>EPVAVVGISCRVPGARDPREFWELLAAGGQAVTDVPADRWNAGDFYDPDRSAPGRSNSRWGGFIEDVDRFDAAFFGISPREAAEMDPQQRLALELGWEALERAGIDPSSLTGTRTGVFAGAIWDDYATLKHRQGGAAITPHTVTGLHRGIIANRLSYTLGLRGPSMVVDSGQSSSLVAVHLACESLRRGESELALAGGVSLNLVPDSIIGASKFGGLSPDGRAYTFDARANGYVRGEGGGFVVLKRLSRAVADGDPVLAVIRGSAVNNGGAAQGMTTPDAQAQEAVLREAHERAGTAPADVRYVELHGTGTPVGDPIEAAALGAALGTGRPAGQPLLVGSVKTNIGHLEGAAGIAGLIKAVLAVRGRALPASLNYETPNPAIPFEELNLRVNTEYLPWEPEHDGQRMVVGVSSFGMGGTNAHVVLEEAPGVVEGASVVESTVGGSAVGGGVVPWVVSAKSAAALDAQIERLAAFASRDRTDGVDAGAVDAGAVDAGAVARVLAGGRAQFEHRAVVVGSGPDDLAAALAAPEGLVRGVASGVGRVAFVFPGQGTQWAGMGAELLDSSAVFAAAMAECEAALSPYVDWSLEAVVRQAPGAPTLERVDVVQPVTFAVMVSLARVWQHHGVTPQAVVGHSQGEIAAAYVAGALSLDDAARVVTLRSKSIAAHLAGKGGMLSLALSEDAVLERLAGFDGLSVAAVNGPTATVVSGDPVQIEELARACEADGVRARVIPVDYASHSRQVEIIESELAEVLAGLSPQAPRVPFFSTLEGAWITEPVLDGGYWYRNLRHRVGFAPAVETLATDEGFTHFVEVSAHPVLTMALPGTVTGLATLRRDNGGQDRLVASLAEAWANGLAVDWSPLLPSATG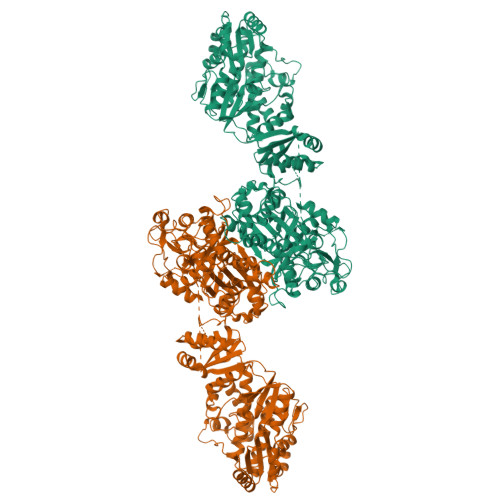HHSDLPTYAFQTERHWL[2x]> DPVEDGLVIETDSGPVEIVTKTAPPAFLADTFDTIYSGWHFRDDSTRDLERDDFDNPA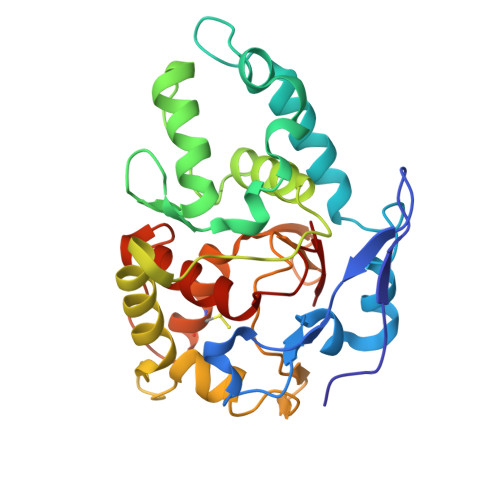MVFVDRGLDKWNAAMGVNGESCASCHQGPESMAGLRAVMPRVDEHTGKLMIMEDYVNACVTERMGLEKWGVTSDNMKDMLSLISLQSRGMAVNVKIDGPAAPYWEHGKEIYYTRYGQLEMSCANCHEDNAGNMIRADHLSQGQINGFPTYRLKDSGMVTAQHRFVGCVRDTRAETFKAGSDDFKALELYVASRGNGLSVEGVSVRH> MGSSHHHHHHSQDPMLYKGDTLYLDWLEDGIAELVFDAPGSVNKLDTATVASLGEAIGVLEQQSDLKGLLLRSNKAAFIVGADITEFLSLFLVPEEQLSQWLHFANSVFNRLEDLPVPTIAAVNGYALGGGCECVLATDYRLATPDLRIGLPETKLGIMPGFGGSVRMPRMLGADSALEIIAAGKDVGADQALKIGLVDGVVKAEKLVEGAKAVLRQAINGDLDWKAKRQPKLEPLKLSKIEATMSFTIAKGMVAQTAGKHYPAPITAVKTIEAAARFGREEALNLENKSFVPLAHTNEARALVGIFLNDQYVKGKAKKLTKDVETPKQAAVLGAGIMGGGIAYQSAWKGVPVVMKDINDKSLTLGMTEAAKLLNKQLER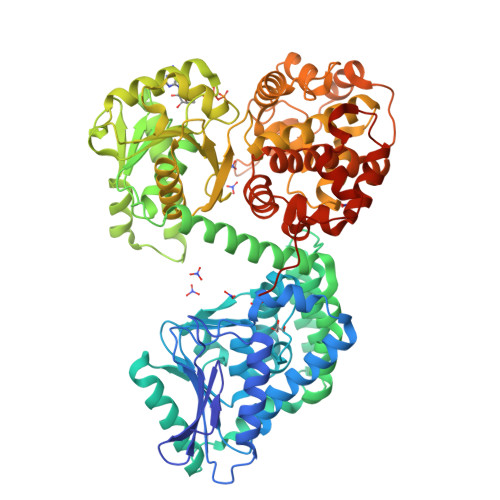GKIDGLKLAGVISTIHPTLDYAGFDRVDIVVEAVVENPKVKKAVLAETEQKVRQDTVLASNTSTIPISELANALERPENFCGMHFFNPVHRMPLVEIIRGEKSSDETIAKVVAWASKMGKTPIVVNDCPGFFVNRVLFPYFAGFSQLLRDGADFRKIDKVMEKQFGWPMGPAYLLDVVGIDTAHHAQAVMAAGFPQRMQKDYRDAIDALFDANRFGQKNGLGFWRYKEDSKGKPKKEEDAAVEDLLAEVSQPKRDFSEEEIIARMMIPMVNEVVRCLEEGIIATPAEADMALVYGLGFPPFHGGAFRWLDTLGSAKYLDMAQQYQHLGPLYEVPEGLRNKARHNEPYYPPVEPARPVGDLKTA> PVIQTFVSTPLDHHKRENLAQVYRAVTRDVLGKPEDLVMMTFHDSTPMHFFGSTDPVACVRVEALGGYGPSEPEKVTSIVTAAITKECGIVADR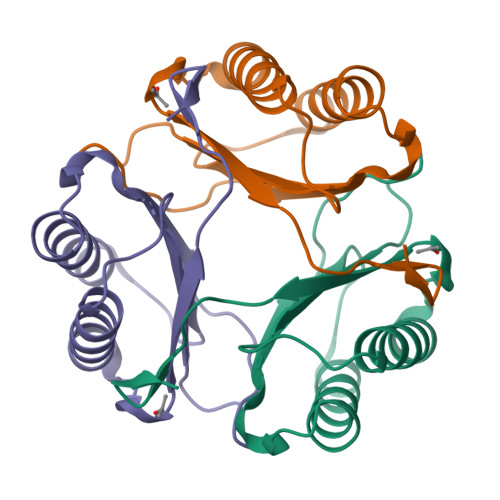IFVLYFSPLHCGWNGTNF> GGSMADKEKAEGNKFYKARQFDEAIEHYNKAWELHKDITYLNNRAAAEYEKGEYETAISTLNDAVEQGREMRADYKVISKSFARIGNAYHKLGDLKKTIEYYQKSLTEHRTADILT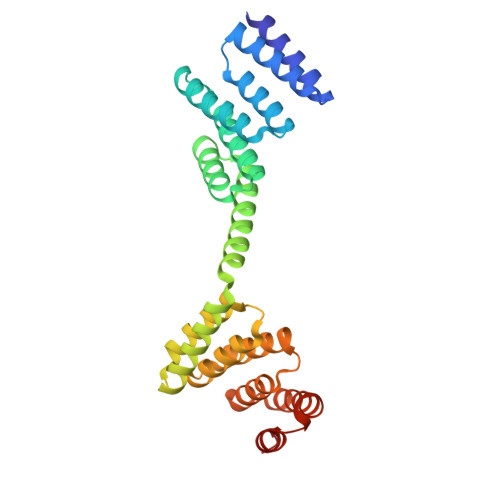KLRNAEKELKKAEAEAYVNPEKAEEARLEGKEYFTKSDWPNAVKAYTEMIKRAPEDARGYSNRAAALAKLMSFPEAIADCNKAIEKDPNFVRAYIRKATAQIAVKEYASALETLDAARTKDAEVNNGSSAREIDQLYYKASQ>[2x]MHHHHHHGENLYFQGSAPYASLTEIEHLVQSVCKSYRETCQLRLEDLLRQRSNIFSREEVTGYQRKSMWEMWERCAHHLTEAIQYVVEFAKRLSGFMELCQNDQIVLLKA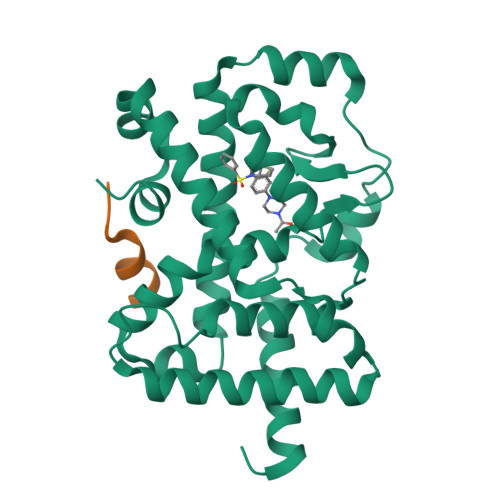GAMEVVLVRMCRAYNADNRTVFFEGKYGGMELFRALGCSELISSIFDFSHSLSALHFSEDEIALYTALVLINAHRPGLQEKRKVEQLQYNLELAFHHHLCKTHRQSILAKLPPKGKLRSLCSQHVERLQIFQHLHPIVVQAAFPPLYKELFSTE;>[2x]AHKILHRLLQE>[2x]SNAQQAIVHNNCQDTVYVQSFPYDGSATGPLTTLQAGQTFSEDFRKSGSTVKVSKTKTLTSPMFIGY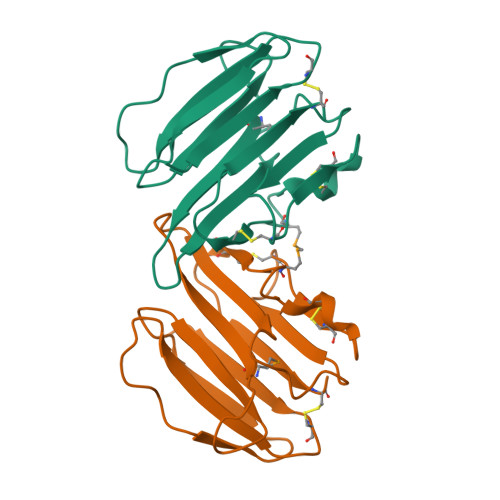SFSSNPDYGYYELSSEWGNPFADKRVTLSPGAGCQDFNCAPNDAGCYSRPDMKKVYGCPLPINVEATLCA>GQNHHEVVKFMDVYQRSYCHPIETLVDIFQEYPDEIEYIFKPSCVPLMRCGGCCNDEGLECVPTEESNITMQIMRIKPHQGQHIGEMSFLQHNKCECRPKKD[2x];>RG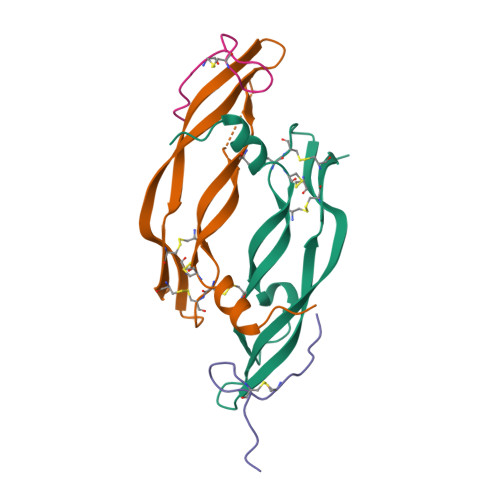WVEICAADDYGRCLTEAQ[2x]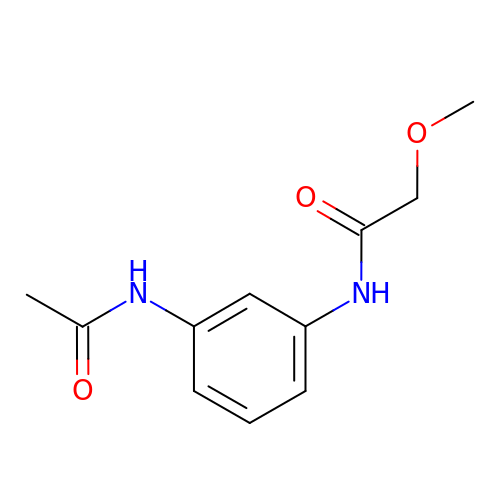~{N}-(3-acetamidophenyl)-2-methoxy-ethanamide | C11 H14 N2 O3 | ZDALGCTWWSVNDR-UHFFFAOYSA-N3-chloranyl-4-pyridin-4-yl-1H-pyrrole-2-carboxamide 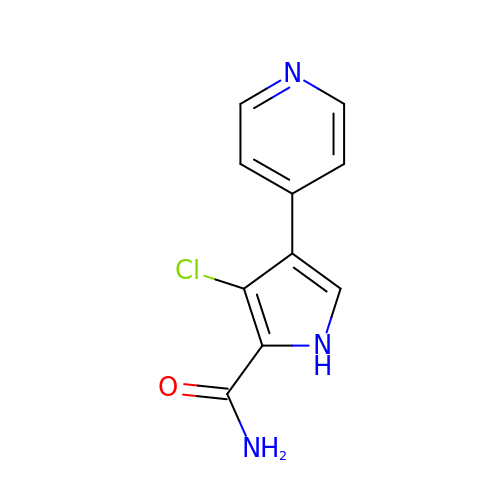| C10 H8 Cl N3 O | PGLBZRZEQTVNDN-UHFFFAOYSA-N>[2x]MSLRNDATNAAGAVGAAMRDHILLPAQEMAKLGKS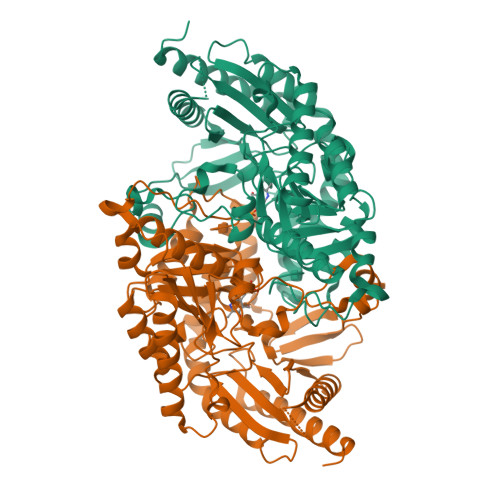AQPVLTHAEGIYVHTEDGRRLIDGPAGMWCAQVGYGRREIVDAMAHQAMVLPYASPWYMATSPAARLAEKIATLTPGDLNRIFFTTGGSTAVDSALRFSEFYNNVLGRPQKKRIIVRYDGYHGSTALTAACTGRTGNWPNFDIAQDRISFLSSPNPRHAGNRSQEAFLDDLVQEFEDRIESLGPDTIAAFLAEPILASGGVIIPPAGYHARFKAICEKHDILYISDEVVTGFGRCGEWFASEKVFGVVPDIITFAKGVTSGYVPLGGLAISEAVLARISGENAKGSWFTNGYTYSNQPVACAAALANIELMEREGIVDQAREMADYFAAALASLRDLPGVAETRSVGLVGCVQCLLDPTRADGTAEDKAFTLKIDERCFELGLIVRPLGDLCVISPPLIISRAQIDEMVAIMRQAITEVSAAHGLTAKEPAAVEGHHHHHH> 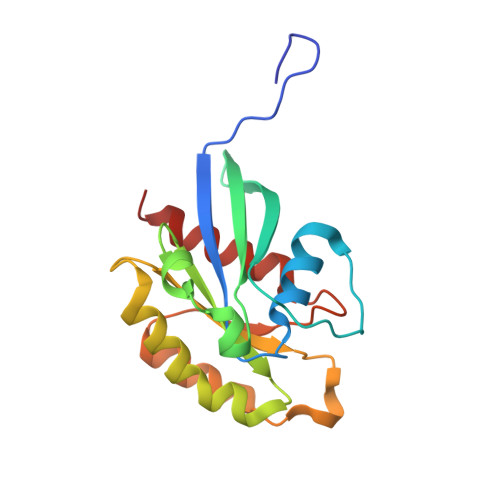GPLGSMSSMNPEYDYLFKLLLIGDSGVGKNCLLLRFADDTYTESYISTIGVDFKIRTIELDGKTIKLQIWDTAGQERFRTITSSYYRGAHGIIVVYDVTDQESFNNVKQWLQEIDRYASENVNKLLVGNKCDLTTKKVVDYTTAKEFADSLGIPFLETSAKNATNVEQSFMTMAAEIKKRM>MRSFVLLAFTLSLLAGCSSGPRLNTDYTSANQDSRVQFIVLHYTSTDLPHSLGILTHGGVSAHYLIGDDEPATVYRLVDENRRAWHAGVSEWQGRTWLNATSIGIEIVNQGYRDTPQGRVWYPFSEAQIQALIPLLKDIAKRHGITPDRIIGHSDIAPGRKVDPGPLFPWKRLADAGLVPWPKPGELARRLAELNGQLPDVRWFQQQLARHGYLVPQTGELEKDTRDVIGAFQMKYRPARFDGEPDLETA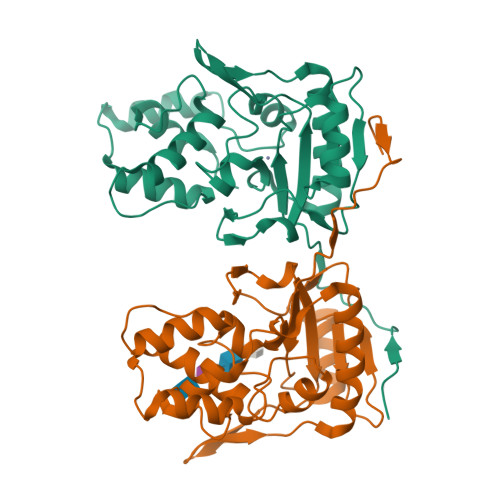ALLLAVPTS[2x]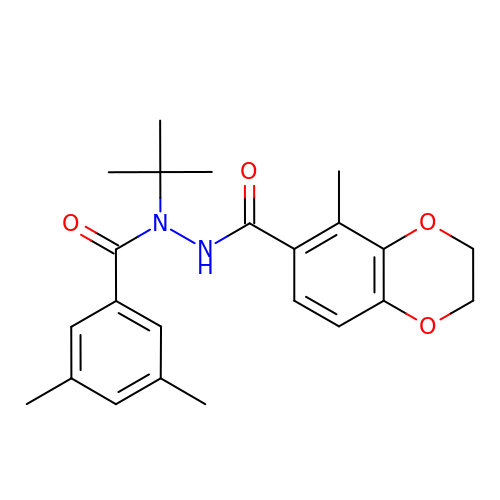N-(TERT-BUTYL)-3,5-DIMETHYL-N'-[(5-METHYL-2,3-DIHYDRO-1,4-BENZODIOXIN-6-YL)CARBONYL]BENZOHYDRAZIDE | C23 H28 N2 O4 | JGJACZABNQGPMT-UHFFFAOYSA-N>FSCNVDGGSSIGAGTTSVYVNLDPVIQPGQNLVVDLSQHISCWNDYGGWYDTDHINLVQGSAFAGSLQSYKGSLYWNNVTYPFPLTTNTNVLDIGDKTPMPLPLKLYITPVGAAGGVVIKAGEVIARIHMYKIATLGSGNPRNFTWNIISN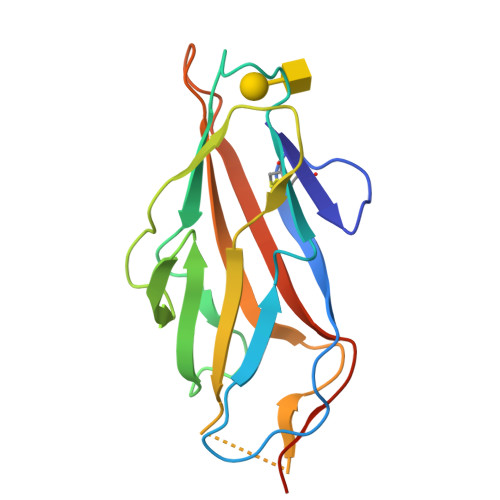NSVVMPTHHHHHH[2x]>GSPGIQSEKGPFVQHINRYLGDDPFLKQFLPLDPHSNQLYELVKDGVLLCKLINVAVPGTIDERAINTKRVLNPWERNENHTLCLNSAKAVGCSVVNIGTQDLAEGRPHLVLGLISQLIKIQLLADLNLKKTPQLVELLEDSDDVEELLRLPPEKVLLKWMNFHLKKGGYKKTVSNFSADLKDAQAYAFLLNVLAPEHCDPATLDAKDPLERAELVLSHAERMNCKRYLTAEEIVEGSSTLNLAFVAQIFHERNGLNKDGKYAFAEMMTEDVETCRDERCYRLWINSLGIDSYVNNVFEDVRNGWILLEVLDKVSPSSVNWKHASKPPIKMPFRKVENCNQVIKIGKQLKFSLVNVAGNDIVQGNKKLILGLLWQLMRFHMLQLLKSLRSRTLGKEMTDADILSWANRKVRTMGRKLQIESFKDKSLSSGLFFLNLLWAVE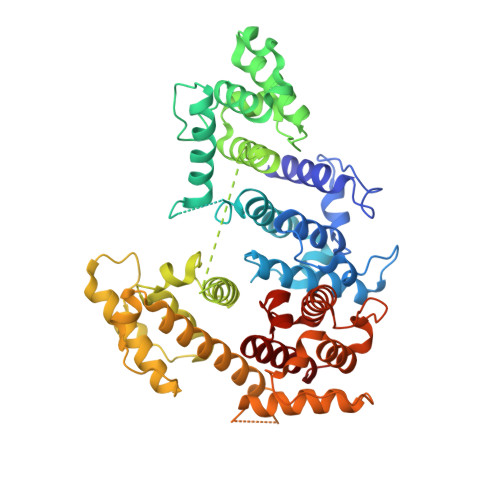PRVVNWNLVTKGETDDEKRLNATYIVSVARKLGCSVFLLPEDIVEVNQKMILILTASIMYWSLQR[2x]> ANTSSAYNSVYDFLRYHDRGDGLTVNGKTSYSIDQAAAQITRENVSWNGTNVFGKSANLTFKFLQSVSSIPSGDTGFVKFNAEQIE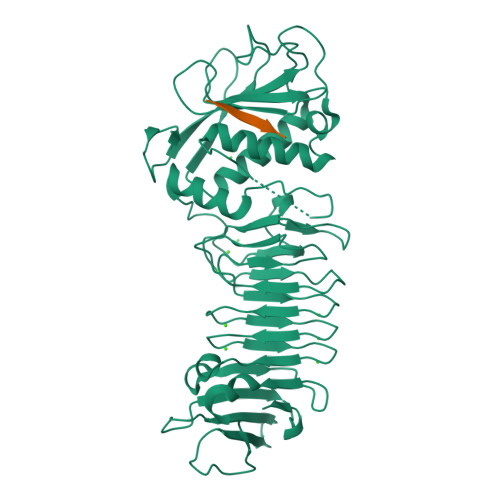QAKLSLQSWSDVANLTFTEVTGNKSANITFGNYTRDASGNLDYGTQAYAYYPGNYQGAGSSWYNYNQSNIRNPGSEEYGRQTFTHEIGHALGLAHPGEYNAGEGDPSYNDAVYAEDSYQFSIASYWGENETGADYNGHYGGAPMIDDIAAIQRLYGANMTTRTGDSVYGFNSNTDRDFYTATDSSKALIFSVWDAGGTDTFDFSGYSNNQRINLNEGSFSDVGGLKGNVSIAHGVTIENAIGGSGNDILVGNSADNILQGGAGNDVLYGGAGADTLYGGAGRDTFVYGSGQDSTVAAYDWIADFQKGIDKIDLSAFRNEGQLSFVQDQFTGKGQEVMLQWDAANSITNLWLHEAGHSSVDFLVRIVGQAAQSDIIV;> AEAAQA(1R,2R,3S,4R,6S)-4,6-diamino-2,3-dihydroxycyclohexyl 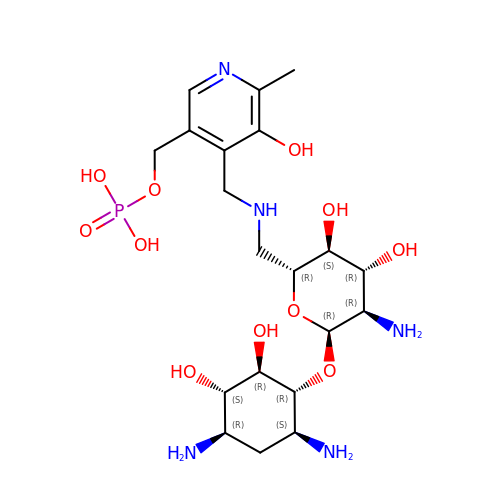2-amino-2,6-dideoxy-6-[({3-hydroxy-2-methyl-5-[(phosphonooxy)methyl]pyridin-4-yl}methyl)amino]-alpha-D-glucopyranoside | C20 H36 N5 O11 P | YAANPRCSTYUZOJ-GMRNZWOESA-N>[2x]SNKCDVVVVGGGISGM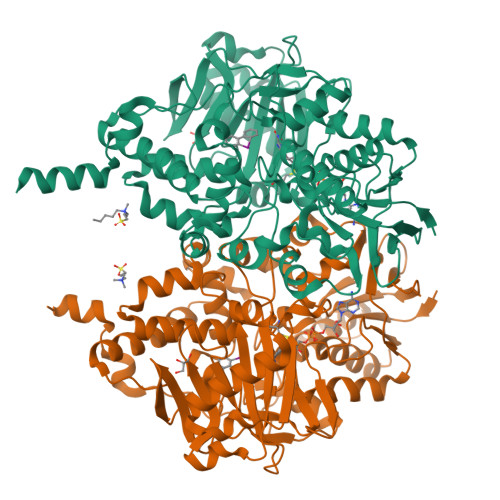AAAKLLHDSGLNVVVLEARDRVGGRTYTLRNQKVKYVDLGGSYVGPTQNRILRLAKELGLETYKVNEVERLIHHVKGKSYPFRGPFPPVWNPITYLDHNNFWRTMDDMGREIPSDAPWKAPLAEEWDNMTMKELLDKLCWTESAKQLATLFVNLCVTAETHEVSALWFLWYVKQCGGTTRIISTTNGGQERKFVGGSGQVSERIMDLLGDRVKLERPVIYIDQTRENVLVETLNHEMYEAKYVISAIPPTLGMKIHFNPPLPMMRNQMITRVPLGSVIKCIVYYKEPFWRKKDYCGTMIIDGEEAPVAYTLDDTKPEGNYAAIMGFILAHKARKLARLTKEERLKKLCELYAKVLGSLEALEPVHYEEKNWCEEQYSGGCYTTYFPPGILTQYGRVLRQPVDRIYFAGTETATHWSGYMEGAVEAGERAAREILHAMGKIPEDEIWQSEPESVDVPAQPITTTFLERHLPSVPGLLRLIGLTTIFSATALGFLAHKRGLLVRV> FDCGKPQVEPKKCPGRVVGGCVAHPHSWPWQVSLRTRFGMHFCGGTLISPEWVLTAAHCLEKSPRPSSYKVILGAHQEVNLEPHVQEIEVSRLFLEPTRKDIALLKLSSPAVITDKVIPACLPSPNYVVADRTECFITGWGETQGTFGAGLLKEAQLPVIENKVCNRYEFLNGRVQSTE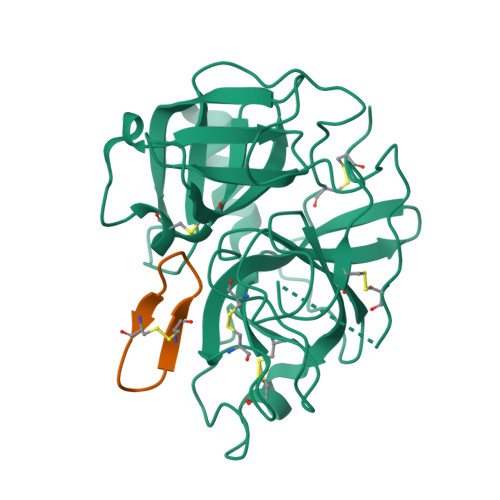LCAGHLAGGTDSCQGDAGGPLVCFEKDKYILQGVTSWGLGCARPNKPGVYVRVSRFVTWIEGVMRNN;> GRCYKSRPPICFPN> MKTTPLVHVASVEKGRSYEDF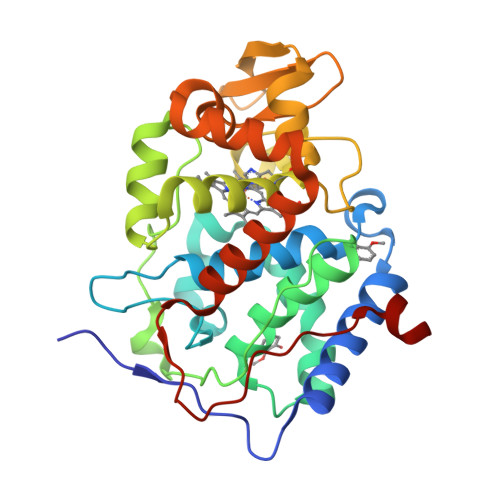QKVYNAIALKLREDDEYDNAIGYGPVLVRLAWHTSGTWDKHDNTGGSYGGTYRFKKEFNDPSNAGLQNGFKFLEPIHKEFPWISSGDLFSLGGVTAVQEMQGPKIPWRCGRVDTPEDTTPDNGRLPDADKDADYVRTFFQRLNMNDREVVALMGAHALGKTHLKRSGYEGPWGAANNVFTNEFYLNLLNENWKLEKNDANNEQWDSKSGYMMLPTDYSLIQDPKYLSIVKEYANDQDKFFKDFSKAFEKLLENGITFPKDAPSPFIFKTLEEQGL>[2x]NSPHSRAMYVYPPNVESSPELPKHIYNKLDKGQIIVVIWVIVSPNNDKQKYTLKINH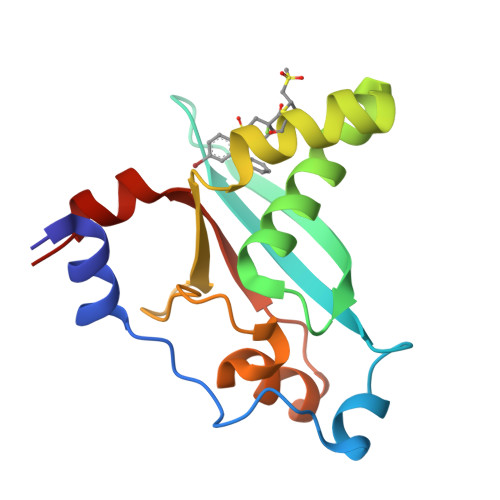DCVPEQVIAEAIRKKTRSMLLSSEQLKLCVLEYQGKYILKVCGCDEYFLEKYPLSQYKYIRSCIMLGRMPNLMLMAKESLYSQLPMD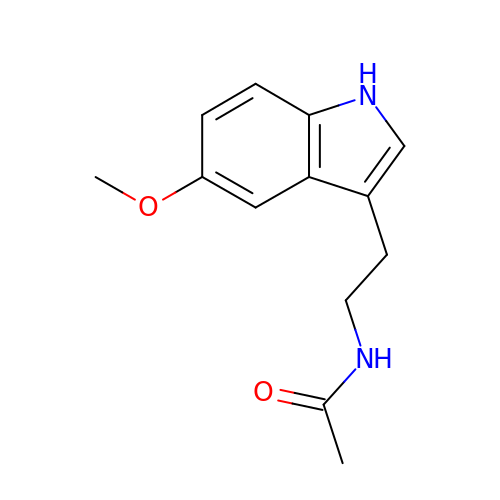N-[2-(5-methoxy-1H-indol-3-yl)ethyl]acetamide | C13 H16 N2 O2 | DRLFMBDRBRZALE-UHFFFAOYSA-N>[6x]GAMGALQGCRSVEEFQCLNRIEEGTYGVVYRAKDKKTDEIVALKRLKMEKEKEGFPITSLREINTILKAQHPNIVTVREIVVGSNMDKIYIVMNYVEHDLKSLMETMKQPFLPGEVKTLMIQLLRGVKHLHDNWILHRDLKTSNLLL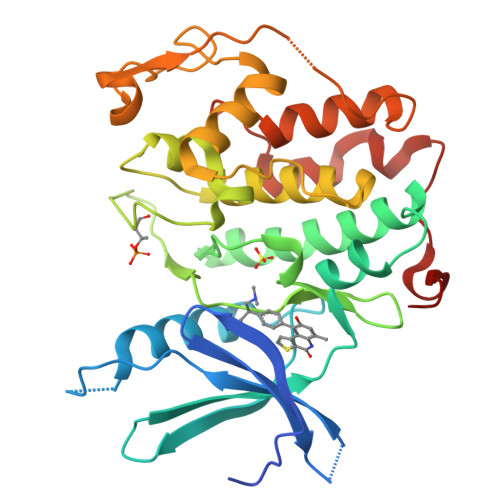SHAGILKVGDFGLAREYGSPLKAYTPVVVTLWYRAPELLLGAKEYSTAVDMWSVGCIFGELLTQKPLFPGKSEIDQINKVFKDLGTPSEKIWPGYSELPAVKKMTFSEHPYNNLRKRFGALLSDQGFDLMNKFLTYFPGRRISAEDGLKHEYFRETPLPIDPSMFPKLVEKY> APMKLYGAVMSWNLTRCATALEEAGSDYEIVPINFATAEHKSPEHLVRNPFGQVPALQDGDLYLFESRAICKYAARKNKPELLREGNLEEAAMVDVWIEVEANQYTAALNPILFQVLISPMLGGTTDQKVVDENLEKLKKVLEVYEARLTKCKYLAGDFLSLADLNHVSVTLCLFA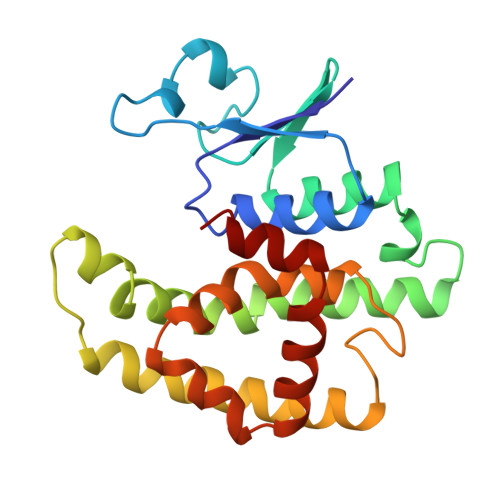TPYASVLDAYPHVKAWWSGLMERPSVQKVAALM> EYERRIAARF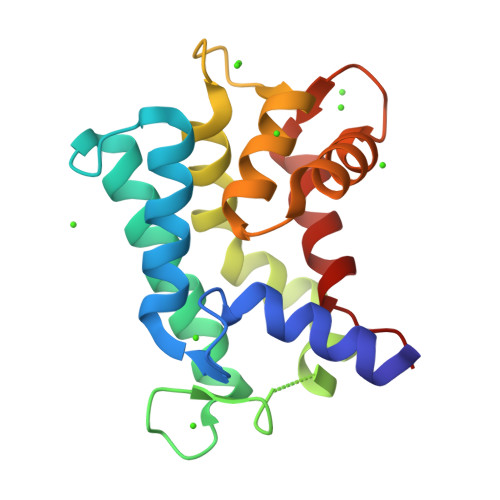TTFDQDGNGHIDRSDFSGAAKALLAEFGVAARSDRGQALYGGAEALWQGLAGIADRDGDQRITREEFVTGAVKRLRDKPDRFAEIARPFLHAALGVADTDGDGAVTVADTARALTAFGVPEDLARQAAAALDTDGDGKVGETEIVPAFARYFTVPA>[2x]KFE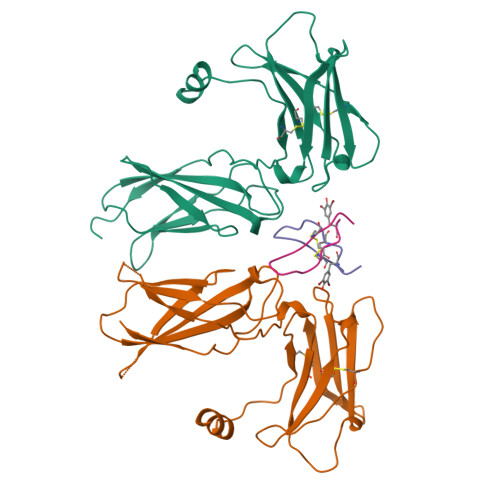SKAALLAARGPEELLCFTERLEDLVCFWEEAASAGVGPGNYSFSYQLEDEPWKLCRLHQAPTARGAVRFWCSLPTADTSSFVPLELRVTAASGAPRYHRVIHINEVVLLDAPVGLVARLADESGHVVLRWLPPPETPMTSHIRYEVDVSAGNGAGSVQRVEILEGRTECVLSNLRGRTRYTFAVRARMAEPSFGGFWSAWSEPVSLLTPSDL;>GGTYSCHFGPLTWVCKPQGG[2x]> ELTPDQQTLLHFIMDSYNKQRMPQEITNKILKEEFSAEENFLILTEMATNHVQVLVEFTKKLPGFQTLDHEDQIALLKGSAVEAMFLRSAEIFNKKLPSGHSDLLEERIRNSGISDEYITPMFSFYKSIGELKMTQEEYALLTAIVILSPDRQYIKDREAVEKLQ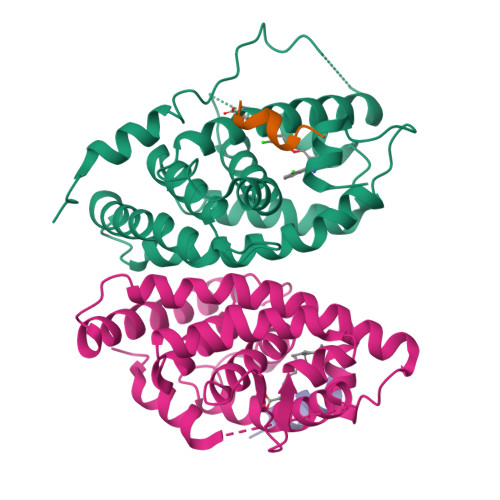EPLLDVLQKLCKIHQPENPQHFAELLGRLTELRTFNHHHAEMLMSWRVNDHKFTPLLEEIWDVQ;>[2x]ERHKILHRLLQEGSPS;> SANEDMPVERILEAELAVEPKTETYVEANMGLNPSSPNDPVTNICQAADKQLFTLVEWAKRIPHFSELPLDDQVILLRAGWNELLIASFSHRSIAVKDGILLATGLHVHRNSAHSAGVGAIFDRVLTELVSKMRDMQMDKTELGCLRAIVLFNPDSKGLSNPAEVEALREKVYASLEAYCKHKYPEQPGRFAKLLLRLPALRSIGLKCLEHLFFFKLIGDTPIDTFLMEMLEAPHQMT Even though the composition of the replication machineries may differ between archaea, eukaryotes and bacteria, all use DNA dependent DNA polymerases (DNA pols) for the replication of the genome. In various studies, it was reported that the archaeal B-family DNA polymerases accept a broader range of modified nucleotide triphosphates as substrate than the bacterial A-family DNA pols. We report the first crystal structures of archaeal B-family DNA pols (KOD and 9°N) complexed with primer, template and incoming dNTP in the active site in a state just prior to catalysis. As both DNA pols are similar in sequence (sequence identity 27.4%) and structure (RMSD of 0.689 over 599 Cα atoms) we describe the KOD DNA pol structure in the following and only mention the 9°N DNA pol structure in cases of significant differences.

Ternary 9°N crystals were prepared similar to the KOD crystals. The crystals containing two or three divalent metal ions in the active site were harvested from the same crystallization drop. In addition, we obtained a structure of 9°N DNA pol in complex with dATP and also three metal ions bound in the active site. The three metal ions show the same coordination as observed for KOD DNA pol, with Mg2+ occupying the third metal binding site in 9°N DNA pol. Metal ion A (Mg2+, green) is coordinated by two water molecules, D542, the α-phosphate of the dATP (pink) and D404. Metal ion B (Mn2+, purple) is coordinated by the α-, β- and γ-phosphate, D404, F405 and D542. Metal ion C (Mg2+, green) is coordinated by the γ-phosphate, E580, F405, D404 and three water molecules, whereof one molecule is coordinated by E578 and the other by K464 of the finger domain (yellow). The dATP makes further direct contacts with conserved residues of the finger domain (yellow), N491, K487 and R460 as well as a water mediated contact to K464. The coordinating amino acid side chains show the exact same coordination in both polymerases. Here, the third metal ion is believed to affect the incorporation of either right or wrong nucleotides, thereby modulating the catalytic efficiency. This third metal ion is also present in the complexes of KOD and 9°N DNA pols, which show a similar coordination as observed in DNA pol δ.

> MILDTDYITENGKPVIRVFKKENGEFKIEYDRTFEPYFYALLKDDSAIEDVKKVTAKRHGTVVKVKRAEKVQKKFLGRPIEVWKLYFNHPQDVPAIRDRIRAHPAVVDIYEYDIPFAKRYLIDKGLIPMEGDEELTMLAFAIATLYHEGEEFGTGPILMISYADGSEARVITWKKIDLPYVDVVSTEKEMIKRFLRVVREKDPDVLITYNGDNFDFAYLKKRCEELGIKFTLGRDGSEPKIQRMGDRFAVEVKGRIHFDLYPVIRRTINLPTYTLEAVYEAVFGKPKEKVYAEEIAQAWESGEGLERVARYSMEDAKVTYELGREFFPMEAQLSRLIGQSLWDVSRSSTGNLVEWFLLRKAYKRNELAPNKPDERELARRRGGYAGGYVKEPERGLWDNIVYLDFRSLYPSIIITHNVSPDTLNREGCKEYDVAPEVGHKFCKDFPGFIPSLLGDLLEERQKIKRKMKATVDPLEKKLLDYRQRAIKILANSFYGYYGYAKARWYCKECAESVTAWGREYIEMVIRELEEKFGFKVLYADTDGLHATIPGADAETVKKKAKEFLKYINPKLPGLLELEYEGFYVRGFFVTKKKYAVIDEEGKITTRGLEIVRRDWSEIAKETQARVLEAILKHGDVEEAVRIVKEVTEKLSKYEVPPEKLVIHEQITRDLRDYKATGPHVAVAKRLAARGVKIRPGTVISYIVLKGSGRIGDRAIPADEFDPTKHRYDAEYYIENQVLPAVERILKAFGYRKEDLRYQKTKQVGLGAWLKVKGKK Here we report the mechanism of three Fe(II)/α-ketoglutarate-dependent dioxygenases in bicyclomycin synthesis, which depicts the natural tactic to sequentially hydroxylate specific C−H bonds of similar substrates (cyclodipeptides). Three αKGDs (BcmE/BcmC/BcmG) catalyze site- and stereo-selective hydroxylation of inert C−H bonds in BCM’s (bicyclomycin) cyclic dipeptide scaffold (Fig. 1b3), one of the simplest peptide derivatives without additional functional groups. Our hypothesis posits distinct regulatory mechanisms: BcmE employs steric hindrance, BcmC relies on inherent reactivity, while BcmG utilizes a directing group to control C–H hydroxylation. Although these three enzymes share only 35–42% amino acid identities, the overall structures are similar, and r.m.s.d. values are 0.70 Å (SsBcmE vs SsBcmC), 1.07 Å (SsBcmE vs PaBcmG) and 0.87 Å (SsBcmC vs PaBcmG), respectively.

To investigate the effect of the microenvironment of these three enzymes on the site selectivity, we attempted to determine the crystal structures of SsBcmE, SsBcmC, and SsBcmG from Streptomyces sapporonensis. Despite the extensive screening, we only obtained the binary or ternary complexes crystals of SsBcmE and SsBcmC, with Fe(II) or/and αKG, but failed for that of SsBcmG. As a result, we determined a collection of X-ray crystal structures including ternary complexes of SsBcmE, SsBcmC, PaBcmG (with Fe(II) or/and αKG).

>[3x]VSTETLRLQKARATEEGLAFETPGGLTRALRDGCFLLAVPPGFDTTPGVTLCREFFRPVEQGGESTRAYRGFRDLDGVYFDREHFQTEHVLIDGPGRERHFPPELRRMAEHMHELARHVLRTVLTELGVARELWSEVTGGAVDGRGTEWFAANHYRSERDRLGCAPHKDTGFVTVLYIEEGGLEAATGGSWTPVDPVPGCFVVNFGGAFELLTSGLDRPVRALLHRVRQCAPRPESADRFSFAAFVNPPPTGDLYRVGADGTATVARSTEDFLRDFNERTWGDGYADFGIAPPEPAGVAEDGVRALEHHHHHHHH>[2x]MDAAQQGDTTTILMLPWLGYGHLSAFLELAKSLSRRNFHIYFCSTSVNLDAIKPKLPSSFSDSIQFVELHLPSSPEFPPHLHTTNGLPPTLMPALHQAFSMAAQHFESILQTL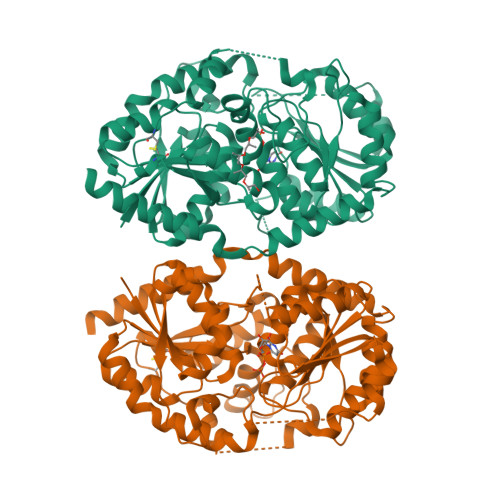APHLLIYDSLQPWAPRVASSLKIPAINFNTTGVFVISQGLHPIHYPHSKFPFSEFVLHNHWKAMYSTADGASTERTRKRGEAFLYCLHASCSVILINSFRELEGKYMDYLSVLLNKKVVPVGPLVYEPNQDGEDEGYSSIKNWLDKKEPSSTVFVSFGSEYFPSKEEMEEIAHGLEASEVNFIWVVRFPQGDNTSGIEDALPKGFLERAGERGMVVKGWAPQAKILKHWSTGGFVSHCGWNSVMESMMFGVPIIGVPMHVDQPFNAGLVEEAGVGVEAKRDPDGKIQRDEVAKLIKEVVVEKTREDVRKKAREMSEILRSKGEEKFDEMVAEISLLLKIEHHHHHH> MNLIPTVIEQTSRGERAYDIYSRLLKDRIIMLGSAIDDNVANSIVSQLLFLDAQDPEKDIFLYINSPGGSISAGMAIYDTMNFVKADVQTIGMGMAAAMGSFLLTAGANGKRFALPNAEIMIHQPLGGAQGQATEIEIAARHILKIKERMNTIMAEKTGQPYEVIARDTD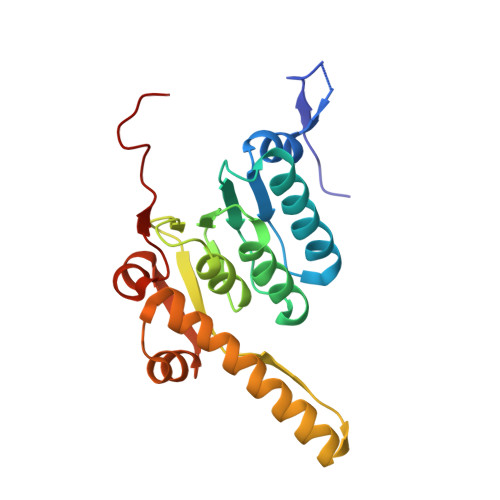RDNFMTAQEAKDYGLIDDIIINKSGLKG> MAAQGFLLIATFLLVLMVLARPLGSGLARLINDIPLPGTTGVERVLFRALGVSDREMNWKQYLCAILGLNMLGLAVLFFMLLGQHYLPLNPQQLPGLSWDLALNTAVSFVTNTNWQSYSGETTLSYFSQMAGLTVQNFLSAASGIAVIFALIRAFTRQSMSTLGNAWVDLLRITLWVLVPVALLIALFFIQQGALQNFLPYQAVNTVEGAQQLLPMGPVASQEAIKMLGTNDGGFFNANSSHPFENPTALTNFVQMLAIFLIPTALCFAFGEVMGDRRQGRMLLWAMSVIFVICVGVVMWAEVQGNPHLLALGTDSSINMEGKESRFGVLVSSLFAVVTTAASCGAVIAMHDSFTALGGMVPMWLMQIGEVVFGGVGSGLYGMMLFVLLAVFIAGLMIGRTPEYLGKKIDVREMKLTALAILVTPTLVLMGAALAMMTDAGRSAMLNPGPHGFSEVLYAVSSAANNNGSAFAGLSANSPFWNCLLAFCMFVGRFGVIIPVMAIAGSLVSKKSQAASSGTLPTHGPLFVGLLIGTVLLVGALTFIPALALGPVAEYLS;> MSRKQLALFEPTLVVQALKEAVKKLNPQAQWRNPVMFIVWIGSLLTTCISIAMASGAMPGNALFSAAISGWLWITVLFANFAEALAEGRSKAQANSLKGVKKTAFARKLREPKYGAAADKVPADQLRKGDIVLVEAGDIIPCDGEVIEGGASVDESAITGEAAPVIRESGGDFASVTGGTRILSDWLVIECSVNPGETFLDRMIAMVEGAQRRKTPNEIALTILLIALTIVFLLATATLWPFSAWGGNAVSVTVLVALLVCLIPTTIGGLLSAIGVAGMSRMLGANVIATSGRAVEAAGDVDVLLLDKTGTITLGNRQASEFIPAQGVDEKTLADAAQLASLADETPEGRSIVILAKQRFNLRERDVQSLHATFVPFTAQSRMSGINIDNRMIRKGSVDAIRRHVEANGGHFPTDVDQKVDQVARQGATPLVVVEGSRVLGVIALKDIVKGGIKERFAQLRKMGIKTVMITGDNRLTAAAIAAEAGVDDFLAEATPEAKLALIRQYQAEGRLVAMTGDGTNDAPALAQADVAVAMNSGTQAAKEAGNMVDLDSNPTKLIEVVHIGKQMLMTRGSLTTFSIANDVAKYFAIIPAAFAATYPQLNALNIMCLHSPDSAILSAVIFNALIIVFLIPLALKGVSYKPLTASAMLRRNLWIYGLGGLLVPFIGIKVIDLLLTVCGLV;> MSGLRPALSTFIFLLLITGGVYPLLTTVLGQWWFPWQANGSLIREGDTVRGSALIGQNFTGNGYFHGRPSATAEMPYNPQASGGSNLAVSNPELDKLIAARVAALRAANPDASASVPVELVTASASGLDNNITPQAAAWQIPRVAKARNLSVEQLTQLIAKYSQQPLVKYIGQPVVNIVELNLALDKLDE;> MSAGVITGVLLVFLLLGYLVYALINAE

KdpFABC (K+-dependent P-type ATPase) is a K+ pump that is responsible for high-affinity electrogenic K+ uptake into prokaryotes at very low extracellular K+ concentrations. The heterotetrameric complex combines a P-type ATPase (KdpB) with a channel-like subunit (KdpA) from the superfamily of K+ transporters (SKT). The channel-like subunit KdpA consists of four nonidentical, covalently linked membrane-pore-membrane (MPM) motifs, referred to as domains 1–4 (D1–D4), which are arranged in a pseudo-four-fold symmetrical pore. KdpB is a 7-TM P-type ATPase.

To this end, we determined cryo-EM structures of the complex loaded with K+ and Rb+, both arrested in an E1·ATP state. To incorporate Rb+, we employed variant KdpFAG232DBS162AC, in which a central glycine (KdpAG232) of the KdpA SF is mutated to allow passage of Rb+9. K+ ions co-purified in the intersubunit tunnel of the variant were exchanged for Rb+ by applying turnover conditions. Here, the KdpBS162A mutation prevented the inhibitory phosphorylation in the A domain, enabling turnover. In both samples, the complex was trapped by the addition of the nonhydrolysable ATP analog AMPPCP prior to cryo-EM sample preparation. The structures were determined at a global resolution of 3.1 and 3.2 Å in the K+- and Rb+-loaded samples, respectively, with higher local resolution in the transmembrane region. Both structures are nearly identical and adopt an E1·ATP conformation. When comparing the individual nonprotein densities in both structures low-pass filtered to the same resolution, the densities in the KdpA SF S3 site and the KdpB CBS are increased ca. two-fold in intensity in the presence of Rb+, close to the expected factor of 2.524–26. This suggests that the densities at both the beginning and the end of the intersubunit tunnel indeed correspond to ions, not waters, and, consequently, that the tunnel constitutes the ion translocation pathway. The nonprotein density in the S1 site is absent in the Rb+-loaded structure, probably because the mutation KdpAG232D changes the SF geometry.>METKHSNRARSRKGALRGAVLAGALMALVGCQTSPAATTSSNTGGTNMQLQLTQEWDKTFPLSAKVEHRKVTFANRYGITLAADLYLPKNRGGDRLPAIVIGGPFGAVKEQSSGLYAQTMAERGFVTLAFDPSYTGESGGQPRNVASPDINTEDFSAAVDFISLLPEVNRERIGVIGICGWGGMALNAVAVDKRVKAVVTSTMYDMTRVMSKGYNDSVTLEQRTRTLEQLGQQRWKDAESGTPAYQPPYNELKGGEAQFLVDYHDYYMTPRGYHPRAVNSGNAWTMTTPLSFMNMPILTYIKEISPRPILLIHGERAHSRY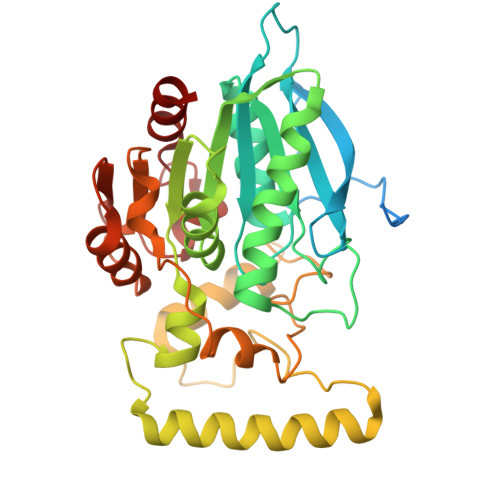FSETAYAAAAEPKELLIVPGASHVDLYDRLDRIPFDRIAGFFDEHL[2x]> MRYIVPIYSFFRSNGLNRFLMIFVLLVIIIPVPMVFIEPEINNYPDAL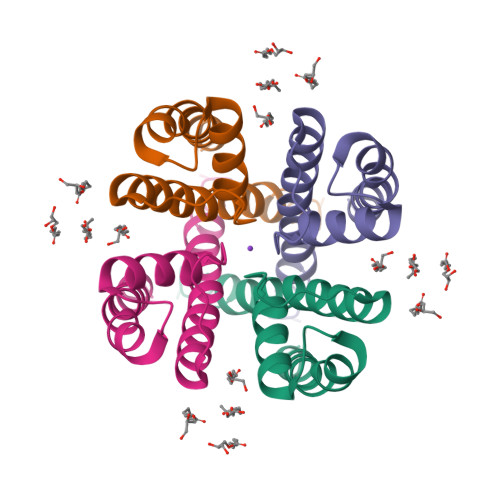WWAIVTATTVGYGDIVPVTPIGRILASIMMLFGIAFIGMITSTITNFFRCKKPTNSSTQRANKITQLISETPDLTKEEIAVVEQFLTLR> QKDANFASGRNSIVHLFEWKWNDIADECERFLQPQGFGGVQISPPNEYLVADGRPWWERYQPVSYI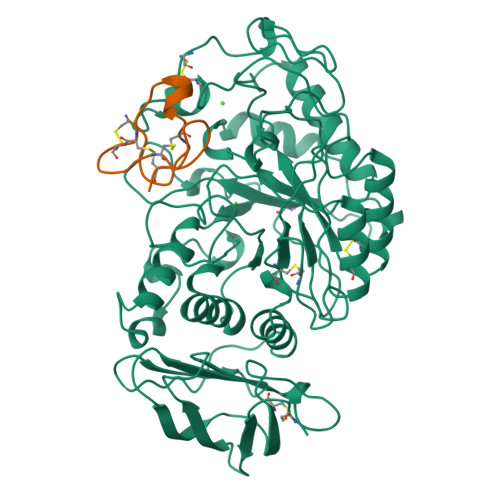INTRSGDESAFTDMTRRCNDAGVRIYVDAVINHMTGMNGVGTSGSSADHDGMNYPAVPYGSGDFHSPCEVNNYQDADNVRNCELVGLRDLNQGSDYVRGVLIDYMNHMIDLGVAGFRVDAAKHMSPGDLSVIFSGLKNLNTDYGFADGARPFIYQEVIDLGGEAISKNEYTGFGCVLEFQFGVSLGNAFQGGNQLKNLANWGPEWGLLEGLDAVVFVDNHDNQRTGGSQILTYKNPKPYKMAIAFMLAHPYGTTRIMSSFDFTDNDQGPPQDGSGNLISPGINDDNTCSNGYVCEHRWRQVYGMVGFRNAVEGTQVENWWSNDDNQIAFSRGSQGFVAFTNGGDLNQNLNTGLPAGTYCDVISGELSGGSCTGKSVTVGDNGSADISLGSAEDDGVLAIHVNAKL;> CIPKWNRCGPKMDGVPCCEPYTCTSDYYGNCS(2R)-2-(2,4-dichlorophenoxy)propanoic acid | C9 H8 Cl2 O3 | 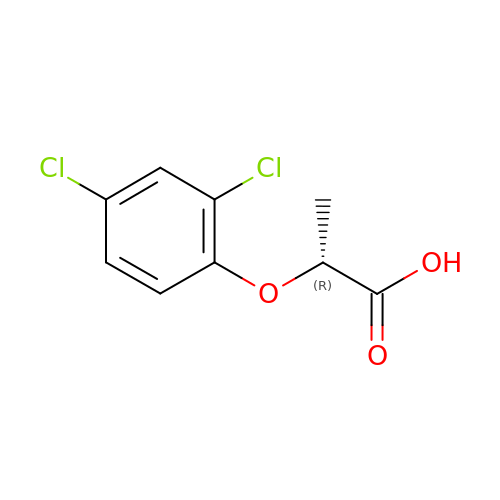MZHCENGPTKEIGP-RXMQYKEDSA-N1-nitrocyclohexene 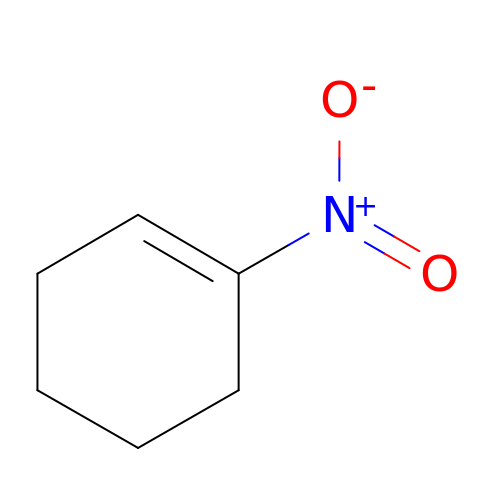| C6 H9 N O2 | DJBRXNRKYAWTBL-UHFFFAOYSA-N> MRRLGVFCRGQRNSPLLTRGIATGGRVTNEDRRWWLVHLECAPDITPGTFIAWL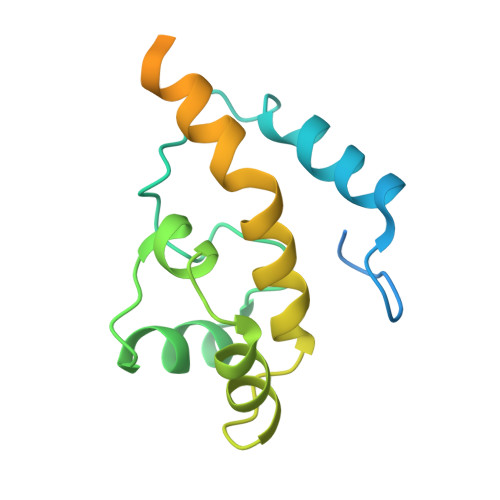DCCGTHTCKKLIERNIWTIEQVAALDSDQVDELKYREGCLKMDVVWEHARTIITPLRQREVTGGVESELQGRIMELRKKRELERRREEILKERANVSEQREETLRK> AAAAAATESDRIAGIFNIPAGIIPTGNVLSTIEVCAHRCIFDFFKQIRSDDNSLYSAQFDILLGTYCNTLNFVRFLELGLSVACICTKFPELAYVRDGVIQFEVQQPMIARDGPHPVDQPVHNYMVKRIHKRSLSAAFAIASEALSLLSNTYVDGTEIDSSLRIRAIQQMARNLRTVLDSFERGTADQLLGVLLEKAPPLSLLSPINKFQPEGHLNRVA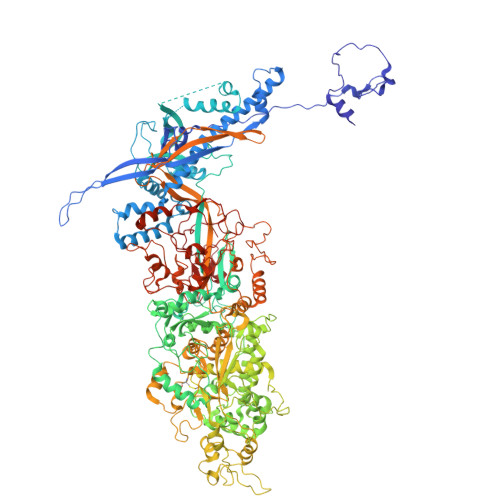RAALLSDLKRRVCADMFFMTRHAREPRLISAYLSDMVSCTQPSVMVSRITHTNTRGRQVDGVLVTTATLKRQLLQGILQIDDTAADVPVTYGEMVLNGANLVTALVMGKAVRSLDDVGRHLLDITDPNTLNIPSIPPQSNSDSTTAGLPVNARVPADLVIVGDKLVFLEALERRVYQATRVAYPLIGNIDITFIMPMGVFQANSMDRYTRHAGDFSTVSEQDPRQFPPQGIFFYNKDGILTQLTLRDAMGTICHSSLLDVEATLVALRQQHLDRQCYFGVYVAEGTEDTLDVQMGRFMETWADMMPHHPHWVNEHLTILQFIAPSNPRLRFELNPAFDFFVAPGDVDLPGPQRPPEAMPTVNATLRIINGNIPVPLCPISFRDCRGTQLGLGRHTMTPATIKAVKDTFEDRAYPTIFYMLEAVIHGNERNFCALLRLLTQCIRGYWEQSHRVAFVNNFHMLMYITTYLGNGELPEVCINIYRDLLQHVRALRQTITDFTIQGEGHNGETSEALNNILTDDTFIAPILWDCDALIYRDEAARDRLPAIRVSGRNGYQALHFVDMAGHNFQRRDNVLIHGRPVRGDTGQAIPITPHHDREWGILSKIYYYIVIPAFSRGSCCTMGVRYDRLYPALQAVIVPEIPADEEAPTTPEDPRHPLHAHQLVPNSLNVYFHNAHLTVDGDALLTLQELMGDMAERTTAILVSSAPDAGAATATTRNMRIYDGALYHGLIMMAYQAYDETIATGTFFYPVPVNPLFACPEHLASLRGMTNARRVLAKMVPPIPPFLGANHHATIRQPVAYHVTHSKSDFNTLTYSLLGGYFKFTPISLTHQLRTGFHPGIAFTVVRQDRFATEQLLYAERASESYFVGQIQVHHHDAIGGVNFTLTQPRAHVDLGVGYTAVCATAALRCPLTDMGNTAQNLFFSRGGVPMLHDNVTESLRRITASGGRLNPTEPLPIFGGLRPATSAGIARGQASVCEFVAMPVSTDLQYFRTACNPRGRASGMLYMGDRDADIEAIMFDHTQSDVAYTDRATLNPWASQKHSYGDRLYNGTYNLTGASPIYSPCFKFFTPAEVNTNCNTLDRLLMEAKAVASQSSTDTEYQFKRPPGSTEMTQDPCGLFQEAYPPLCSSDAAMLRTAHAGETGADEVHLAQYLIRDASPLRGCLPL> DFQGLYAEVKACSSELESLEMELRQQILVNIGKILQDQPSMEALEASLGQGLCSGGQVEPLDGPAGCILECLVLDSGELVPELAAPIFYLL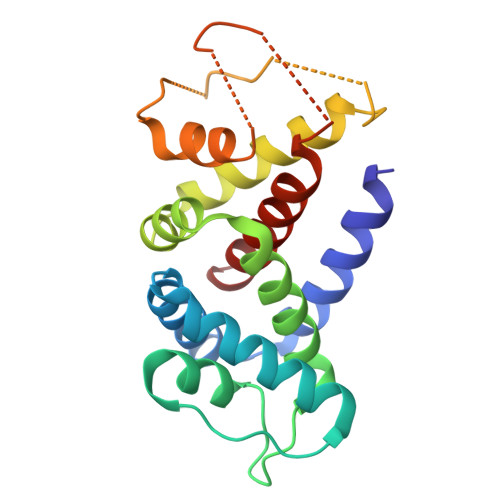GALAVLSETQQQLLAKALETTVLSKQLELVKHVLEQSTPWQEQSSVSLPTVLLGDCWDEKNPTWVLLEECGLRLQVESPQVHWEPTSLIPTSALYASLFLLSSLGQ>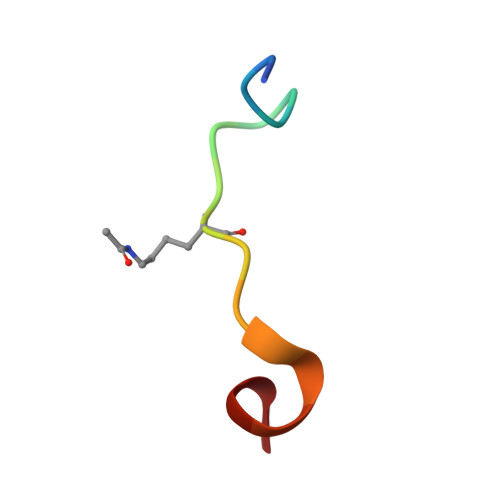 TARKSTGGKAPRKQLAY>[2x]MNLKDSIGLRIKTERERQQMSREVLCLDGAELTVRQLIRIEKGESLPSLDRLSYIAKRLGKSMTELLDQDNITIPDEYYEMKNRLIKFPTYRNPDRIKSKLTLIEEVYEKFFDILPEEELLTLDILENILSFTSWEESPKVEEIYEDLFEQVKRKRKFSTNDLLVIDYYFFHLYGRKQYDKKLFERIIKRVLNQEIWTDDVYNIVLFND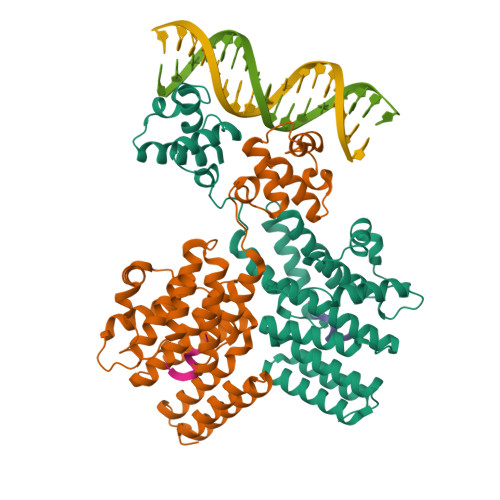LMAIAALKIFHNSFSDFLTVVDKALAVIEKSQLYSYKPSVFVLKAKYELLHKENKKEAAENYDKAIVFASVLEDSVLEESIKAGKLADGLGAGWSHPQFEK;>LPYFAGCL[2x]4-[3-{1-(4-BENZYL)PIPERODINYL}PROPIONYL]-7-METHOXY-2,3,4,5-TERTRAHYDRO-1,4-BENZOTHIAZEPINE | C25 H32 N2 O2 S | 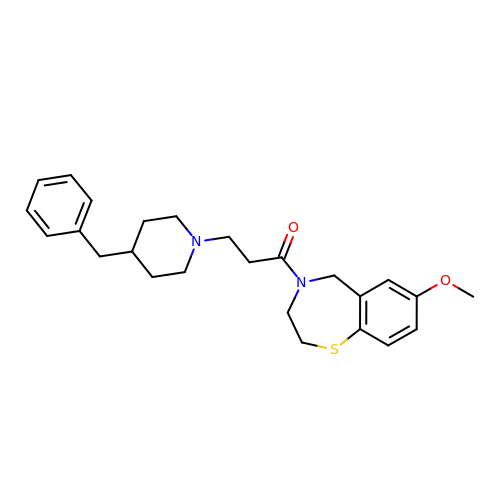KCWGETCFOVJEPI-UHFFFAOYSA-N>HMGRSQNSEFETASDEPIAVIGLSCRLPKASGPQELWQLLDDGASAVTRVPADRETPPSTEEESADGEAAGARWGGFLDRVDTFDAGFFGISPREAAAMDPQQRLVLELSWEALEGAGLVPATLRDTGLGVFVGAARDDYATLYRRREGRAVDHHAMTGLHRSLIANRISYALGAHGPSMVVDTGCSSSLVAVHLACESLRRGESDIALAGGVNLNIAAESARETAAFGGLSPDGQCFTFDARANGFVRGEGGGLVVLKTLRRALADGDLVHGVILASAVNNDGPSDTLTTPSRRAQESLLTRVYRRAGVTPTEVGYVEL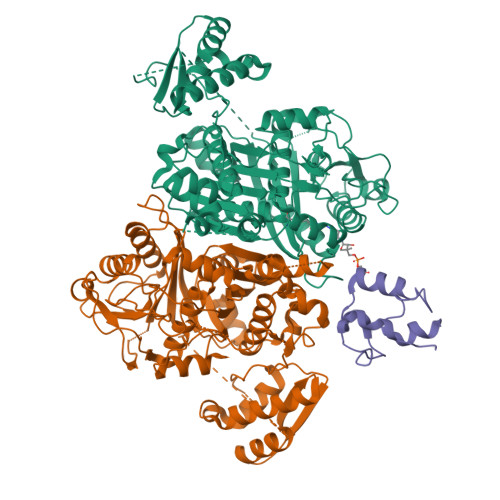HGTGTKVGDPIEAAALGAVLGTGRDTPLPVGSIKTNIGHLEGAAGIAGLIKALLQLRRRRLVPSLNFSTPNPDIPLDALNLRVQQESAPWATPSGGGRTLVAGVSSFGMGGTNCHVVVSAAPVPEDGETTSEAGATGPDSGPALLPWVVSARSPQALRDQAGRLAAWADSPAGREASPVDIGWSLATSRTHFEYRAVVSGSDRDELVASLRALASGSPVTAAGAVDGRAEPVALLSAVGELFADGYPVDWTAYFAGWPAARVELPTYAFQRSRHWLENVPELAVS[2x];> HMPREPVTPDSDHPDPVETVRQLTAHVLGLTAAADVEMTRSFKDLGFDSLMSVELRDRLCAATGLSLATTLLYDHPSPAETAEFVRARLTGDEA>GPMSAQDVENAVEAALDPSVGPIIKQQATDFIGSLRSSSTGWKICHEIFSEKTKYKPSTRLICLQTLSEKVREWNNESNLLELQMIRDSVWSYIKELSFLDEPAYISNAVQHLLTLLFLQLYPSNWNDFFASLQGVIAASSQSEFSNFYLKVLLSIGDEIADSLVLKTDVQIQKDNLVKDAIRANDMSDIVSFVYEMMLAYSNAKNYGTVGLCLQVYAQWVSWININLIVNEPCMNLLYSFLQIEELRCAACETMTEIVNKKMKPLEKLNLLNILNLNLFFSKSQEQSTDPNFDEHVAKLINAQGVELVAIKSDPSELSPELKENCSFQLYNLFPYLIRYLSDDYDETSTAVFPFLSDLLVSLRKESSSKELSASLKEFLKSLLEAIIKKMKYDESQEWDDDPDSEEEAEFQEMRKKLKIFQDTINSIDSSLFSSYMYSAITSSLSTAATLSPENSWQLIEFALYETYIFGEGLRGPDAFFNEVDKSPTVLSQILALVTTSQVCRHPHPLVQLLYMEILVRYASFFDYESAAIPALIEYFVGPRGIHNTNERVRPRAWYLFYRFVKSIKKQVVNYTESSLAMLGDLLNISVSPVTDMDAPVPTLNSSIRNSDFNSQLYLFETVGVLISSGNLTPEEQALYCDSLINALIGKANAALSSDLSALENIISVYCSLMAIGNFAKGFPARGSEEVAWLASFNKASDEIFLILDRMGFNEDIRGAVRFTSGRIINVVGPDMLPKVPQLISILLNSIDMNELVDVLSFISQLIHIYKDNMMEITNRMLPTLLMRIFSSLSAAPQGTDDAVKQNDLRKSYISFILQLLNK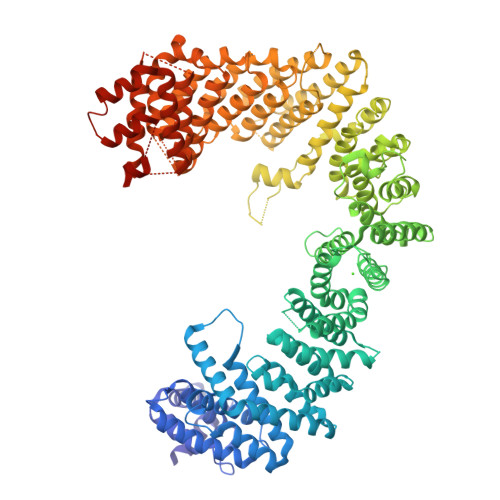GFGSILFTEENQVYFDPLINSILHFANLVGEPATQKSSIALVSKMVSLWGGKDGIAGFENFTLSLTPLCFEMPVNPNFNTRDGQSLVVLGELAGLQKIILEKLGDIYKSYLVTVYFPTVNFPDVMASEYLQALSNLDSRSFKQFFQKFIQALKSGNV[2x]>MASSASGLRRGHP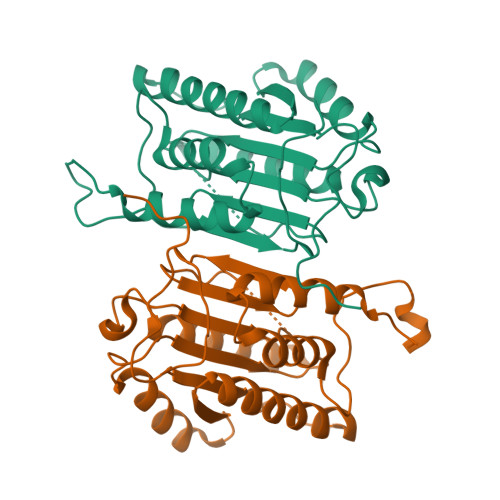AGGEENMTETDAFYKREMFDPAKKYKMDHRRRGIALIFNHERFFWHLTLPERRGTCADRDNLTRRFSDLGFEVKCFNDLKAEELLLKIHEVSTVSHADADCFVCVFLSHGEGNHIYAYDAKIEIQTLTGLFKGDKCHSLVGKPKIFIIQACRGNQHDVPVIPLDVVDNQTEKLDTNITEVDAASVYTLPAGADFLMCYSVAEGYYSHRETVNGSWYIQDLCEMLGKYGSSLEFTELLTLVNRKVSQRRVDFCKDPSAIGKKQVPCFASMLTKKLHFFPKSNLEHHHHHH[4x]Nalpha-[trans-4-(aminomethyl)cyclohexane-1-carbonyl]-N-octyl-O-[(pyridin-4-yl)methyl]-L-tyrosinamide 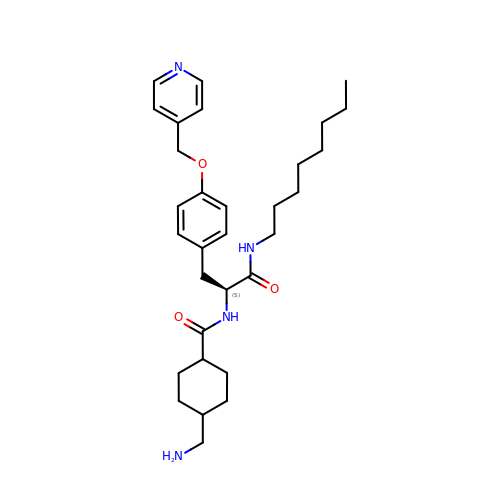| C31 H46 N4 O3 | ZBCXDUNUUKRQSV-RWPDHJIBSA-N>[4x]MREKD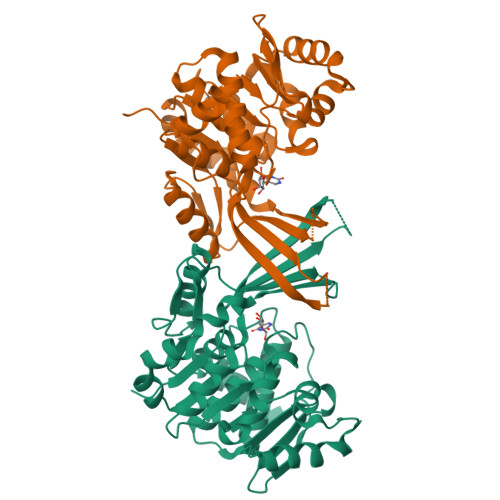YVVIIGSANIDVAGYSHESLNYADANPGKIKFTPGGVGRNIAQNLALLGNKAWLLSAVGSDFYGQSLLTQTNQSGVYVDKCLIVPGENTSSYLSLLDNTGEMLVAINDMNISNAITAEYLAQHREFIQRAKVIVADCNISEEALAWILDNAANVPVFVDPVSAWKCVKVRDRLNQIHTLKPNRLEAETLSGIALSGRDDVAKVAAWFHQHGLNRLVLSMGGDGVYYSDIRGENGWSAPIKTNVINVTGAGDAMMAGLASCWVDGMPFAESVRFAQGCSSMALSCEYTNNPDLSIANVISLVENAECLN[(1S)-1-{[6-(3-chloro-4-methylphenyl)thieno[2,3-d]pyrimidin-4-yl]amino}-2-(3-fluorophenyl)ethyl]phosphonic acid | C21 H18 Cl F N3 O3 P S | 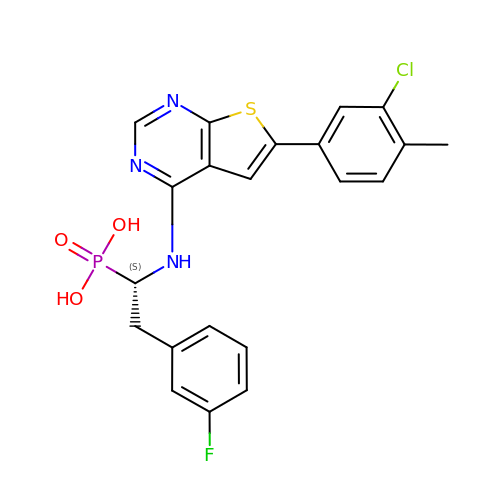ZSPBSSJYWQDARC-IBGZPJMESA-N>GKAFDDGAFTGIREINLSYNKETAIGDFQVVYDLNGSPYVGQNHKSFITGFTPVKISLDFPSEYIMEVSGYTGNVSGYVVVRSLTFKTNKKTYGPYGVTSGTPFNLPIENGLIVGFKGSIGYWLDYFSMYLSL[4x];>D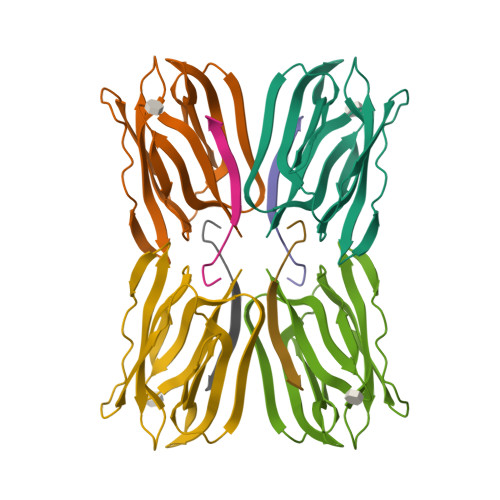EQSGKSQTVIVGPWGAKVS[4x]>[2x]GSHMATFLIKHKAS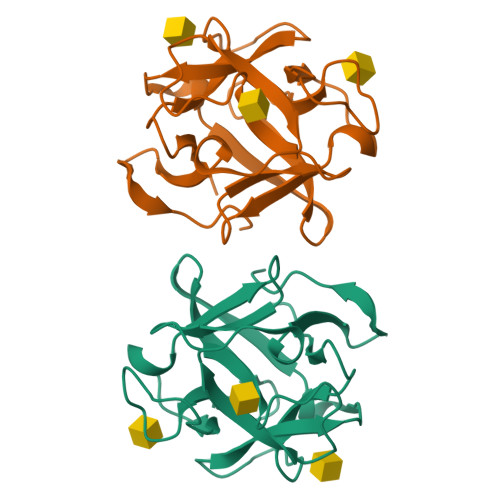GKFLHPKGGSSNPANDTNLVLHSDIHERMYFQFDVVDERWGYIKHAASGKIVHPLGGKADPPNETKLVLHQDRHDRALFAMDFFNDNIIHKAGKYVHPKGGSTNPPNETLTVMHGDKHGAMEFIFVSPKNKDKRVLVYV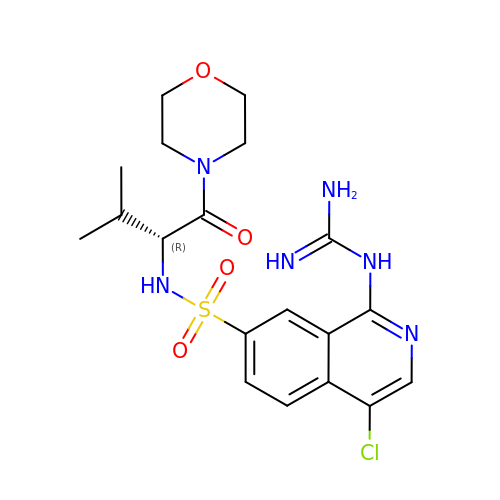1-carbamimidamido-4-chloro-N-[(2R)-3-methyl-1-(morpholin-4-yl)-1-oxobutan-2-yl]isoquinoline-7-sulfonamide | C19 H25 Cl N6 O4 S | JKDPCBXPJMGTJT-MRXNPFEDSA-N> MSPILAHDVVKPQGVAWAFQAKDVENASAP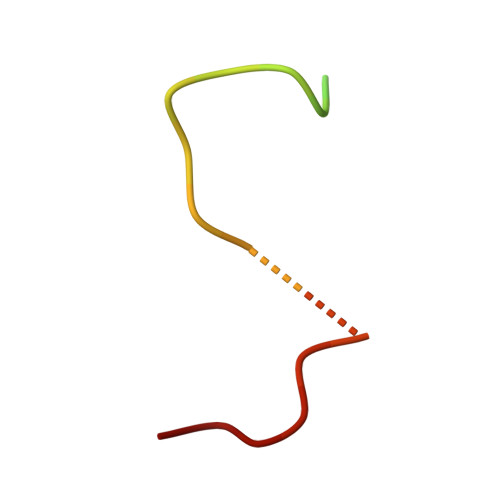V>[2x]MMKFKPNQTRTYDREGFKKRAACLCFRSEQEDEVLLVSSSRYPDQWIVPGGGMEPEEEPGGAAVREVYEEAGVKGKLGRLLGIFENQDRKH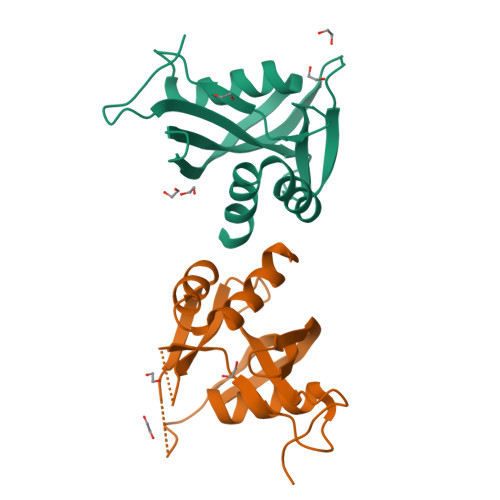RTYVYVLTVTEILEDWEDSVNIGRKREWFKVEDAIKVLQCHKPVHAEYLEKLKLGCSPANGNSTVPSLPDNNALFVTAAQTSGLPSSVR> MNAVLSVQGASAPVKKKSFFSKFTRLNMLRLARAVIPAAVLMMFFPQ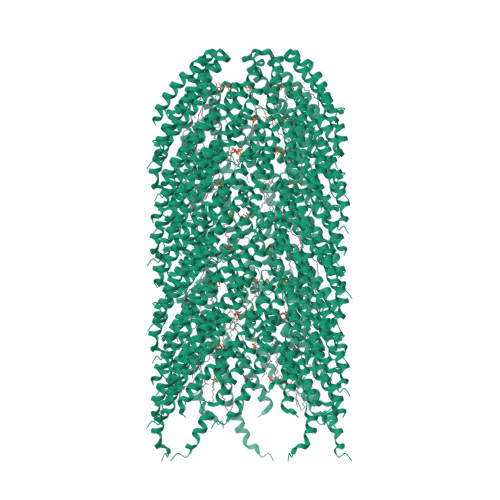LAMAAGSSGQDLMASGNTTVKATFGKDSSVVKWVVLAEVLVGAVMYMMTKNVKFLAGFAIISVFIAVGMAVVGL>[2x]EEGQTGGFSSACTAIDAVYTWVNGSDPNFIEDIRRFDDKYDPSRFDDKNELRYSLRSLEKHAAWIRHVYIVTNGQIPSWLDLSYERVTVVPHEVLAPDPDQLPTFSSSAIETFLHRIPKLSKRFLYLNDDIFLGAPLYPEDLYTEAEGVRVYQAWMVPDCALDCPWTYIGDGACDRHCNIDACQFDGGDCSETGPASDAHVIPPSKEVLEVQPAAVPQSRVHRFPQMGLQKLFRRSSANFKDVMRHRNVSTLKELRRIVERFNKAKLMSLNPELETSSSEPQTTQRHGLRKEDFKSSTDIYSHSLIATNMLLNRAYGFKARHVLAHVGFLIDKDIVEAMQRRFHQQILDTAHQRFRAPTDLQYAFAYYSFLMSETKVMSVEEIFDEFDTDGSATWSDREVRTFLTRIYQPPLDWSAMRYFEEVVQNCTRNLGMHLKVDTVEHSTLVYERYEDSNLPTITRDLV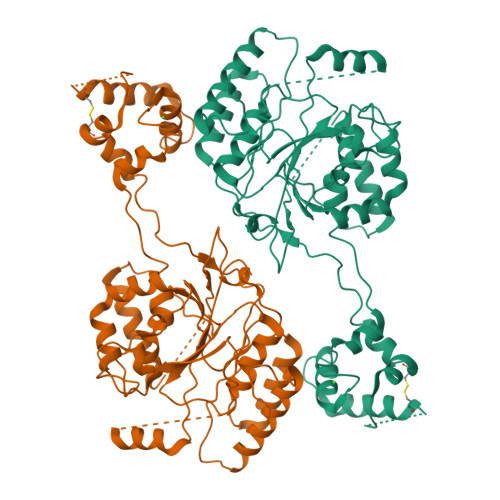VRCPLLAEALAANFAVRPKYNFHVSPKRTSHSNFMMLTSNLTEVVESLDRLRRNPRKFNCINDNLDANRGEDNEMVRHLLEDFYLSFFPRRSKFELPPQYRNRFESWRDFQRWKRRKR>MSDESNPPKVILLVEDSKADSRLVQEVLKTSTIDHELIILRDGLAAMAFLQQQGEYENSPRPNLILLDLNLPKKDGREVLAEIKQNPDLKRIPVVVLTTSHNE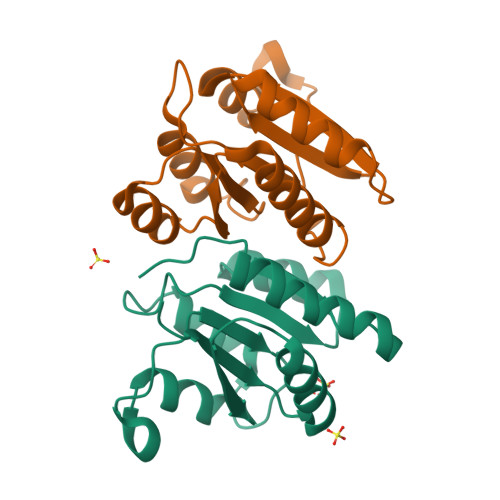DDVIASYELHVNCYLTKSRNLKDLFKMVQGIESFWLETVTLPAA[2x]>[2x]GTQGKVIKCKAAIAWKTGSPLCIEEI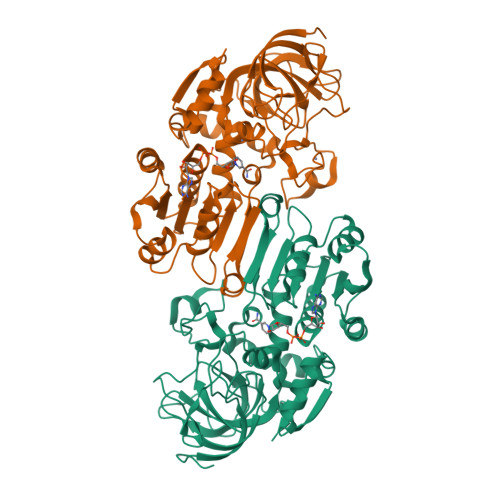EVSPPKACEVRIQVIATCVCPTDINATDPKKKALFPVVLGHECAGIVESVGPGVTNFKPGDKVIPFFAPQCKRCKLCLSPLTNLCGKLRNFKYPTIDQELMEDRTSRFTCKGRSIYHFMGVSSFSQYTVVSEANLARVDDEANLERVCLIGCGFSSGYGAAINTAKVTPGSTCAVFGLGCVGLSAIIGCKIAGASRIIAIDINGEKFPKAKALGATDCLNPRELDKPVQDVITELTAGGVDYSLDCAGTAQTLKAAVDCTVLGWGSCTVVGAKVDEMTIPTVDVILGRSINGTFFGGWKSVDSVPNLVSDYKNKKFDLDLLVTHALPFESINDAIDLMKEGKSIRTILTF> GAHMAGGRSWCLRRVGMSAGWLLLEDGCEVTVGRGFGVTYQLVSKICPLMISRNHCVLKQNPEGQWTIMDNKSLNGVWLNRA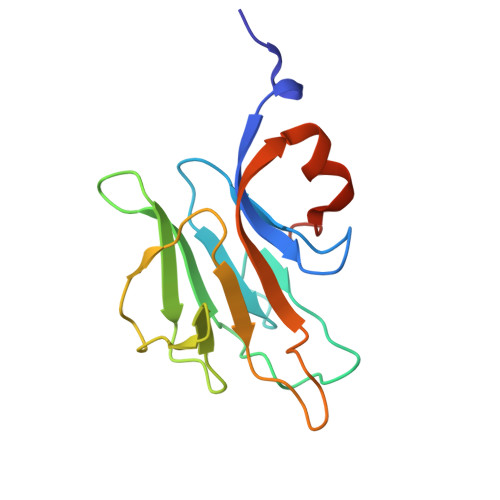RLEPLRVYSIHQGDYIQLGVPLENKENAEYEYEVTEEDWETIYPCLSPKNDQMIEK>[2x]PKKQTRLGLEAKKEENLADWYSQVITKSEMIEYHDISGCYILRPWAYAIWEAIKDFFDAEIKKLGVENCYFPMFVSQSALEKEKTHVADFAPEVAWVTRSGKTELAEPIAIRPTSETVMYPAYAKWVQSHRDLPIKLNQWCNVVRWEFKHPQPFLRTREFLWQEGHSAFATMEEAAEEVLQILDLYAQVYEELLAIPVVKGRKTEKEKFAGGDYTTTIEAFISASGRAIQGGTSHHLGQNFSKMFEIVFEDPKIPGEKQFAYQNSWGLTTRTIGVMTMVHGDNMGLVLPPRVACVQVVIIPCGITNALSEEDKEALIAKCNDYRRRLLSVNIRVRADLRDNYSPGWKFNHWELKGVPIRLEVGPRDMKSCQFVAVRRDTGEKLTVAENEAETKLQAILEDIQVTLFTRASEDLKTHMVVANTMEDFQKILDSGKIVQIPFCGEIDCEDWIKKTTARDQDLEPGAPSMGAKSLCIPFKPLCELQPGAKCVCGKNPAKYYTLFGRSY

Aminoacyl-tRNA synthetases (aaRSs) are an essential enzyme family for protein translation and, in several cases, have been validated drug targets. Among the aaRSs, prolyl-tRNA synthetase (PRS) is a validated drug target in Plasmodial spp and Toxoplasma gondii (Tg). In the current study, we examined five ATP-mimetics L95, L96, L97, L35, and L36, based on the 1-(pyridin-4-yl) pyrrolidin-2-one (PPL) scaffold. We successfully co-crystallized all five compounds with TgPRS (L95, L96, L97, L35, and L36) and three with HsPRS (L95, L96, and L97), all in complex with L-pro.

The complex structure of HsPRS with L95, L96, and L97 was determined to address the structural basis for differential inhibition. Interestingly, co-crystals of HsPRS with these compounds were obtained in two forms, namely forms 1 and 2, in 0.1 M HEPES pH 7.5, 20% PEG 3350 and 0.5 or 1.5 M CaCl2. Form 1 crystals belonged to the monoclinic space group P21 (a = 71, b = 91, c = 83 Å and β = 110°) with two molecules per asymmetric unit, and form 2 crystals belonged to the orthorhombic space group P212121 (a = 70, b = 106, c = 145 Å), except for HsPRS-L97. Significant structural variations within the catalytic domain (1016–1296): ATP pocket (1152–1165), loop (1210–1220), and motif (1084–1115) were observed for the three co-crystallized structures. The loop 1152–1165 exhibited ligand-induced fitting, and the residues Arg1152, Trp1153, Phe1155, Lys1156, and Arg1163 formed a cavity-like structure to fit L95, L96, and L97. These three compounds displayed side-chain rotameric conformational changes relative to the apo-HsPRS shown in Fig 8C. The L-pro pocket exhibited minimal structural and rotameric changes. L-pro was mainly buried within a cavity formed by Glu1123, Phe1167, Trp1169, Glu1171, His1173, Phe1216, His1242, Thr1276, and Arg1278. The active site residues between HsPRS and TgPRS are highly conserved with a few exceptions- His1157 (Gln475), Gln1159 (Thr477), Gly1238 (Ala556), and Gly1239 (Ala557). Similarly, the ΔTm (°C) values for HsPRS were 19, 21, 16, 23, and 10 for L95, L96, L97, L35, and L36, in presence of L-pro, respectively, compared to the apo-HsPRS.(2S)-2-methyl-2,3-dihydrothieno[2,3-f][1,4]oxazepin-5-amine | C8 H10 N2 O S | 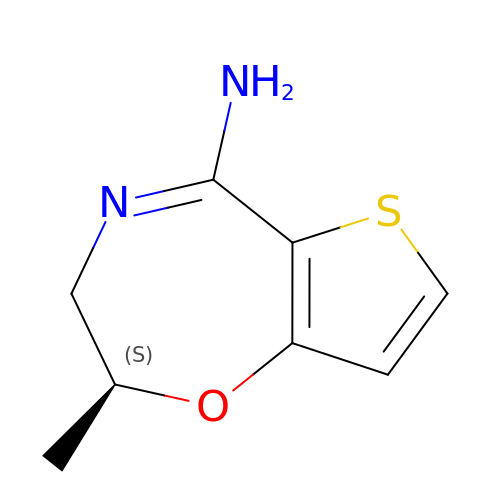TUOXPJFCQDMQOX-YFKPBYRVSA-N> GSHMSYADSSRNAVLTNGGRTLRAE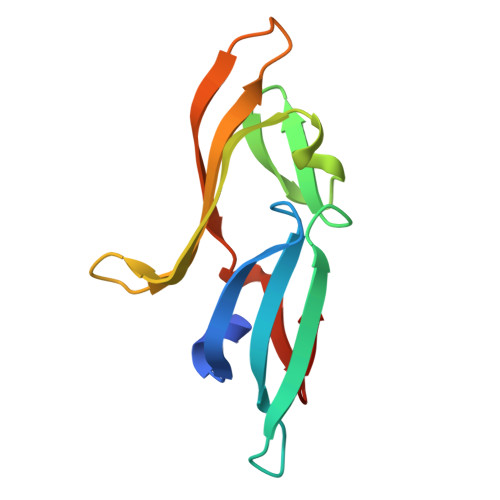CRNADGNWVTSELDLDTIIGNNDGHFQWGGQNFTETAEDIRFHPKEGAAEQPILRARLRDCNGEFHDRDVNLNRIQNVNGRLVFQ(1R,2R,3S,4R,6S)-4,6-DIAMINO-2-[(5-AMINO-5-DEOXY-BETA-D-RIBOFURANOSYL)OXY]-3-HYDROXYCYCLOHEXYL 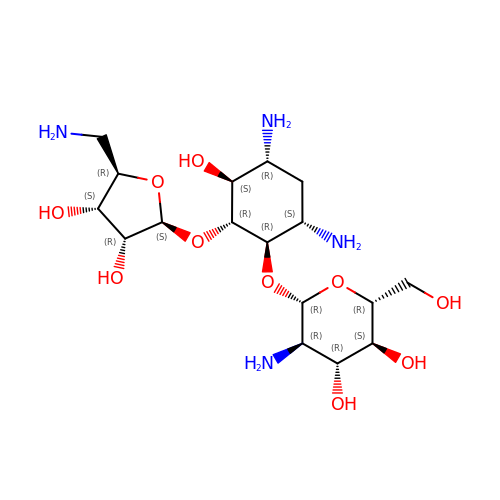2-AMINO-2-DEOXY-ALPHA-D-GLUCOPYRANOSIDE | C17 H34 N4 O10 | FNBQIDOUCINBIA-VVPCINPTSA-N> MSSPSKPTSPFVDDIEHESGSASNGLSSMSPFDDSFQFEKPSSAHGNIEVAKTGGSVLKRQSKPMKDISTPDLSKVTFDGIDDYSNDNDINDDDELNGKKTEIHEHENEVDDDLHSFQATPMPNTGGFEDVELDNNEGSNNDSQADHKLKRVRFGTRRNKSGRIDINRSKTLKWAKKNFHNAIDEFSTKEDSLENS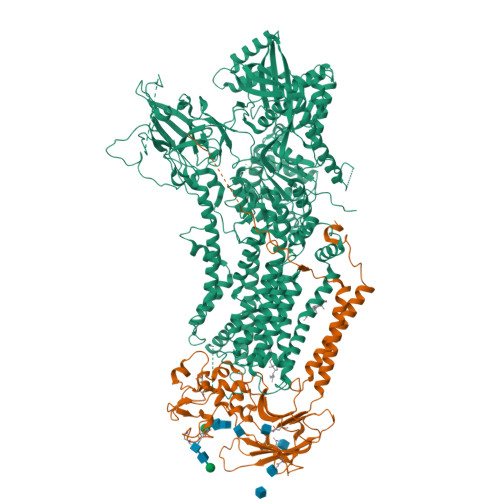ALQNRSDELRTVYYNLPLPEDMLDEDGLPLAVYPRNKIRTTKYTPLTFFPKNILFQFHNFANIYFLILLILGAFQIFGVTNPGFASVPLIVIVIITAIKDGIEDSRRTVLDLEVNNTRTHILSGVKNENVAVDNVSLWRRFKKANTRALIKIFEYFSENLTAAGREKKLQKKREELRRKRNSRSFGPRGSLDSIGSYRMSADFGRPSLDYENLNQTMSQANRYNDGENLVDRTLQPNPECRFAKDYWKNVKVGDIVRVHNNDEIPADMILLSTSDVDGACYVETKNLDGETNLKVRQSLKCSKIIKSSRDITRTKFWVESEGPHANLYSYQGNFKWQDTQNGNIRNEPVNINNLLLRGCTLRNTKWAMGMVIFTGDDTKIMINAGVTPTKKSRISRELNFSVILNFVLLFILCFTAGIVNGVYYKQKPRSRDYFEFGTIGGSASTNGFVSFWVAVILYQSLVPISLYISVEIIKTAQAIFIYTDVLLYNAKLDYPCTPKSWNISDDLGQIEYIFSDKTGTLTQNVMEFKKCTINGVSYGRAYTEALAGLRKRQGVDVESEGRREKEEIAKDRETMIDELRSMSDNTQFCPEDLTFVSKEIVEDLKGSSGDHQQKCCEHFLLALALCHSVLVEPNKDDPKKLDIKAQSPDESALVSTARQLGYSFVGSSKSGLIVEIQGVQKEFQVLNVLEFNSSRKRMSCIIKIPGSTPKDEPKALLICKGADSVIYSRLDRTQNDATLLEKTALHLEEYATEGLRTLCLAQRELTWSEYERWVKTYDVAAASVTNREEELDKVTDVIERELILLGGTAIEDRLQDGVPDSIALLAEAGIKLWVLTGDKVETAINIGFSCNVLNNDMELLVVKASGEDVEEFGSDPIQVVNNLVTKYLREKFGMSGSEEELKEAKREHGLPQGNFAVIIDGDALKVALNGEEMRRKFLLLCKNCKAVLCCRVSPAQKAAVVKLVKKTLDVMTLAIGDGSNDVAMIQSADVGVGIAGEEGRQAVMCSDYAIGQFRYVTRLVLVHGKWCYKRLAEMIPQFFYKNVIFTLSLFWYGIYNNFDGSYLFEYTYLTFYNLAFTSVPVILLAVLDQDVSDTVSMLVPQLYRVGILRKEWNQTKFLWYMLDGVYQSVICFFFPYLAYHKNMVVTENGLGLDHRYFVGVFVTAIAVTSCNFYVFMEQYRWDWFCGLFICLSLAVFYGWTGIWTSSSSSNEFYKGAARVFAQPAYWAVLFVGVLFCLLPRFTIDCIRKIFYPKDIEIVREMWLRGDFDLYPQGYDPTDPSRPRINEIRPLTDFKEPISLDTHFDGVSHSQETIVTEEIPMSILNGEQGSRKGYRVSTTLERRDQLSPVTTTNNLPRRSMASARGNKLRTSLDRTREEMLANHQLDTRYSVERARASLDLPGINHAETLLSQRSRDR;> MVNFDLGQVGEVFRRKDKGAIVSGDNPEEEEDVDASEFEEDEVKPVRTKNRRPKEDAFTQQRLAAINPVLTPRTVLPLYLLIAVVFVIVGGCILAQNSKVDEVTIYYQDCMTNATSSWSDIPSEHWQFVFHKYKTYNTAPQWRFVDDESDDFTKQRGTCQIRFTTPSDMKNNVYLNYVLEKFAANHRRYVLSFSEDQIRGEDASYETVHDATGINCKPLSKNADGKIYYPCGLIANSMFNDTFPLQLTNVGDTSNNYSLTNKGINWESDKKRYKKTKYNYTQIAPPPYWEKMYPDGYNETNIPDIQDWEEFQNWMRPGAFDKITKLIRINKNDTLPAGEYQLDIGLHWPVLEFNGKKGIYLTHGSHLGGRNPFLGIVYLIGGCICAAMALILLTFWLFGGRKIADASSLSWNMK>[2x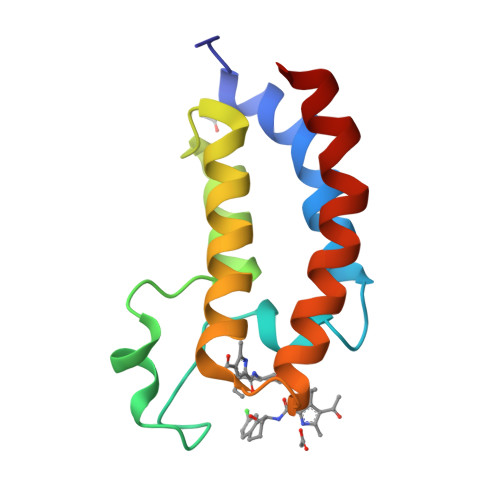]SMIFKPEELRQALMPTLEALYRQDPESLPFRQPVDPQLLGIPDYFDIVKSPMDLSTIKRKLDTGQYQEPWQYVDDIWLMFNNAWLYNRKTSRVYKYCSKLSEVFEQEIDPVMQSLG>[12x]MAFSADTPEIVYTHDTGLDYITYSDYELDPANPLAGGAAWIEGAFVPPSEARISIFDQGFYTSDATYTTFHVWNGNAFRLGDHIERLFSNAESIRLIPPLTQDEVKEIALELVAKTELREAMVTVTITRGYSSTPFERDITKHRPQVYMSA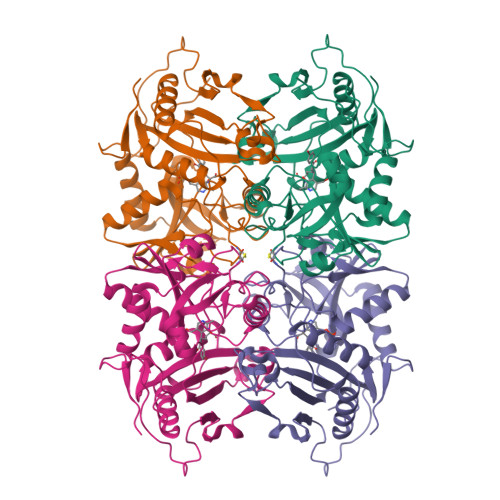CPYQWIVPFDRIRDGVHLMVAQSVRRTPRSSIDPQVKNFQWGDLIRAIQETHDRGFELPLLLDCDNLLAEGPGFNVVVIKDGVVRSPGRAALPGITRKTVLEIAESLGHEAILADITPAELYDADEVLGCSTGGGVWPFVSVDGNSISDGVPGPVTQSIIRRYWELNVEPSSLLTPVQYALE N-METHYL PROTOPORPHYRIN IX 2,4-DISULFONIC 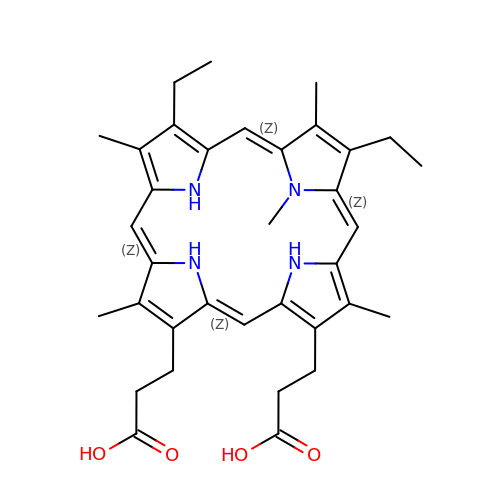ACID | C35 H42 N4 O4 | VIEXPEPYGOTUBM-UQOLDQHFSA-N> SGLQGMDVVHGTATMQVDGNKTIIRNSVDAIINWKQFNIDQNEMVQFLQENNNSAVFNRVTSNQISQLKGILDSNGQVFLINPNGITIGKDAIINTNGFTASTL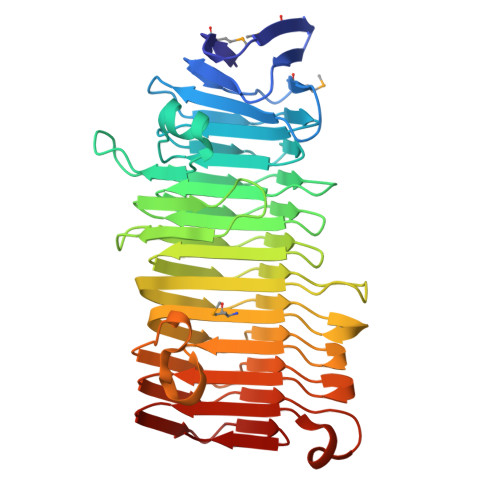DISNENIKARNFTFEQTKDKALAEIVNHGLITVGKDGSVNLIGGKVKNEGVISVNGGSISLLAGQKITISDIINPTITYSIAAPENEAVNLGDIFAKGGNINVRAATIRNQGKLSADSVSKDKSGNIVLSAKEGEAEIGGVISAQNQQAKGGKLMITGDKVTLKTGAVIDLSGKEGGETYLGGDERGEGKNGIQLAKKTSLEKGSTINVSGKEKGGRAIVWGDIALIDGNINAQGSGDIAKTGGFVETSGHDLFIKDNAIVDAKEWLLD> MKFLKNVLEEGSKLEEFNELELSPEDKELLEYLQQTKAKITVVGCGGAGNNTITRLKMEGIEGAKT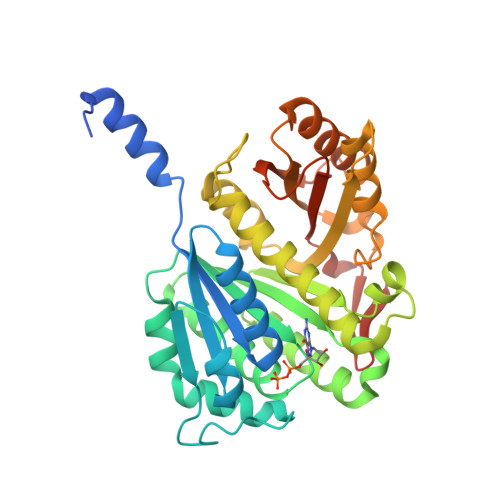VAINTDAQQLIRTKADKKILIGKKLTRGLGAGGNPKIGEEAAKESAEEIKAAIQDSDMVFITCGLGGGTGTGSAPVVAEISKKIGALTVAVVTLPFVMEGKVRMKNAMEGLERLKQHTDTLVVIPNEKLFEIVPNMPLKLAFKVADEVLINAVKGLVELITKDGLINVDFADVKAVMNNGGLAMIGIGESDSEKRAKEAVSMALNSPLLDVDIDGATGALIHVMGPEDLTLEEAREVVATVSSRLDPNATIIWGATIDENLENTVRVLLVITGVQSRIEFTDTGLKRKKLELTGIPKI> TMCYSHTTTSRAILTNCGENSCYRKSRRHPPKM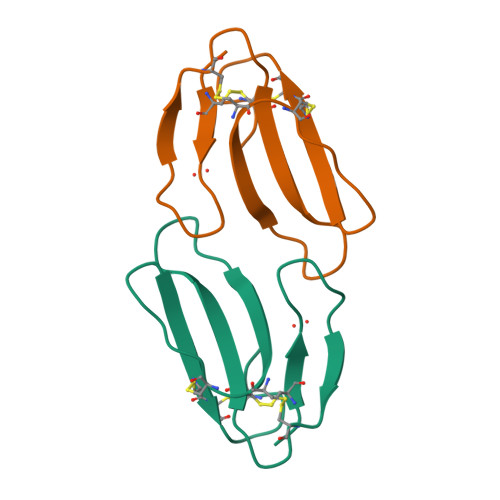VLGRGCGCPPGDDNLEVKCCTSPDKCNY> GSDELLYLPVRGRETYEMLLKIKESLELMQYLPQHTIETYRQQQQQ

The transcription factors p53, p63 and p73 play an important role in cancer prevention, development and longevity. The three proteins share a similar domain organization, being composed of structured DNA-binding domain (DBD) and tetramerization domain flanked by intrinsically disordered regions. Tetramers are formed via a short tetramerization domain that follows the DBD, with a short flexible linker region separating the two domains. Here, we report crystal structures of different p63 tetramerization domain variants, showing not only marked similarity to p73 but also small differences that may be important for regulating the function of p63 in vivo.

We then systematically truncated the C-terminal region, which significantly improved the crystal quality, and we were able to solve the structure of p63(359–402). The crystal structure of the long variant was solved at a resolution of 2.15 Å. The crystals belonged to space group P422 and contained one monomer in the asymmetric unit. Like its family members, p63 forms dimers of dimers with D2 symmetry. The monomers consist of a β-strand followed by two helices, H1 and H2, the latter being absent in the p53 homolog. Tetramers are formed via largely hydrophobic H1–H1 interactions of two primary dimers and H2-mediated contacts. The H2 helices from one primary dimer reach across and clasp the adjacent primary dimer, with the two primary dimers packing in approximately orthogonal fashion via their H1 helices. Helix H2, which is essential for the stability of the tetramer, forms both hydrophobic and polar intersubunit contacts: the latter comprise a hydrogen bond between Tyr396 and Glu383′ and a salt bridge between Arg397 and Glu380′. The last four residues of the construct used for crystallization, Gln399 to Gln402, were not resolved in the crystal structure, indicating a high degree of flexibility.> MGRQWALEDFEIGRPLGKGKFGNVYLAREKQSKFILALKVLFKAQLEKAGVEHQLRREVEIQSHLRHPNILRLYGYFHDATRVYLILEYAPLGTVYRELQKLSKFDEQRTATYITELANALSYCHSKRVIHRDIKPENLLLGSAGELKIADFGWSVHAPSSRRTTLAGTLDYLPPEMIEGRMHDEKVDLWSLGVLCYEFLVGKPPFEANTYQETYKRISRVEFTFPDFVTEGARDLISRLLKHNPSQRPMLREVLEHPWITANSSKPHHHHHH

Aurora A is a serine/threonine protein kinase that plays an important role in controlling early stages of mitosis, including centrosome maturation and separation, mitotic entry, and bipolar spindle formation. Localization and enzymatic activity of Aurora A are regulated by its interaction with the spindle assembly factor TPX2. We have used fragment-based, structure-guided lead discovery to develop small molecule inhibitors of the Aurora A-TPX2 protein–protein interaction (PPI). The initial fragment hits identified from screening with the ATP site blocked by a high-affinity inhibitor were very weakly active, but guided by continuous crystallographic analysis of the inhibitors in complex with Aurora A, we were able to increase target affinity by more than 10,000-fold, clearly demonstrating the ability of fragment-based and structural biology approaches to develop potent PPI inhibitors when a suitable binding pocket is present. These compounds occupy a hydrophobic pocket on the surface of Aurora A, discrete from its ATP-binding catalytic site, which forms the interaction surface for a linear N-terminal segment of the interacting peptide from TPX2.

Through a further iterative development of the inhibitors utilizing the crystal structure-guided drug design and biophysics (FP and ITC), we improved the affinity of our weak, millimolar fragments by over 10,000-fold to generate the lead compound CAM2602. In addition, the meta-channel between Tyr199 and His201 could be further exploited by the replacement of nitrile with heteroaryl ether, to give compounds 9, 10, and the lead compound CAM2602. CAM2602 engages with the Tyr pocket through hydrophobic interactions at the bottom of the pocket and with polar interactions further outside. The indole NH hydrogen bonds with the Glu170 side chain, and the acyl sulfonamide stacks against His201 and Lys166. The pyridine ring in the meta position pushes Tyr199 sideways, creating a channel between His201 and Tyr199 and forming a T-stacked aromatic interaction with the latter. Finally, Arg179 latches on to the central aromatic ring, with CAM2602 bound to a well-defined pocket which is partly induced by the binding of the inhibitor. An overlay of the crystal structures of early hit 2 with CAM2602 bound to Aurora A reveals a remarkable overlap of the core biaryl scaffold in the two compounds. CAM2602 displaces TPX2 from Aurora A with a KD of 19 nM and a ligand efficiency of 0.33. Our lead compound, CAM2602, inhibits Aurora A:TPX2 interaction, binding Aurora A with 19 nM affinity. CAM2602 exhibits oral bioavailability, causes pharmacodynamic biomarker modulation, and arrests the growth of tumor xenografts.>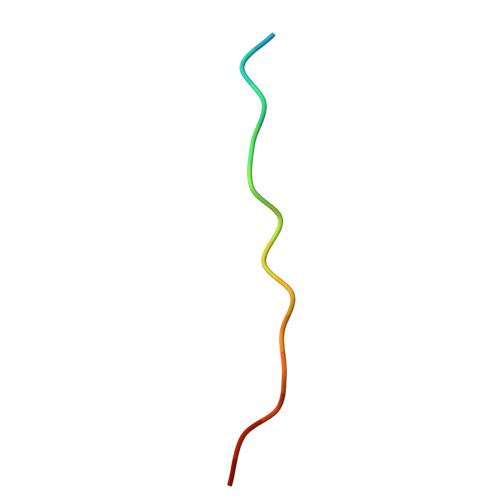 THETGTTNTATTATSN> LPTSNPAQELEARQLGETT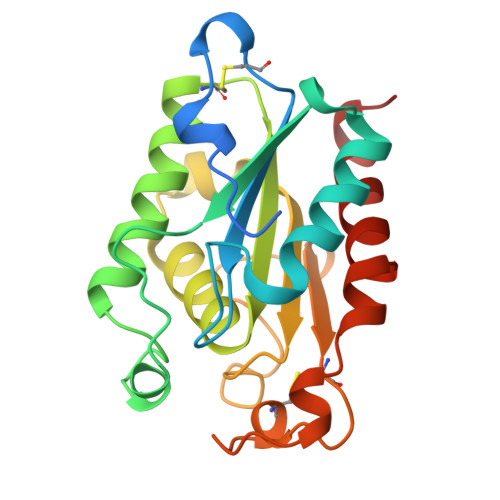RDDLINGNSASCADVIFIYARGSTETGNLGTLGPSIASNLESAFGKDGVWIQGVGGAYRATLGDNALPRGTSSAAIREMLGLFQQANTKCPDATLIAGGYSQGAALAAASIEDLDSAIRDKIAGTVLFGYTKNLQNRGRIPNYPADRTKVFCKTGDLVCTGSLIVAAPHLAYGPDARGPAPEFLIEKVRAVRGSA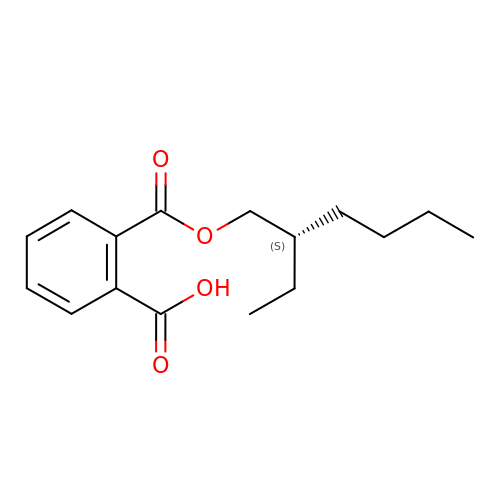2-[(2~{S})-2-ethylhexoxy]carbonylbenzoic acid | C16 H22 O4 | DJDSLBVSSOQSLW-LBPRGKRZSA-N> GPGGEMQKIVFKIPMVDDKSRTKAMSLVASTVGVHSVA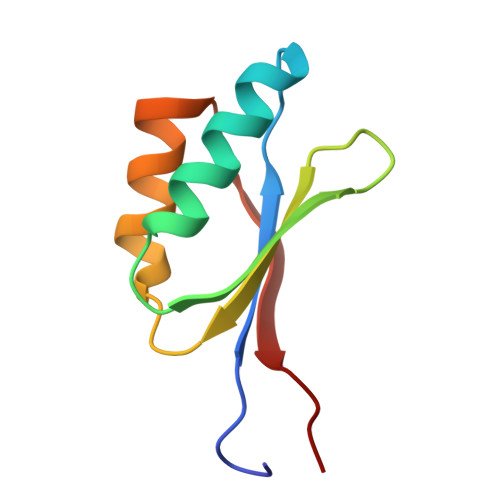IAGDLRDQVVVVGDGIDSINLVSALRKKVGPAMFLEVSQVKED> MAPKAKIVLVGSGMIGGVMATLIVQKNLGDVVLFDIVKNMPHGKALDTSHTNVMAYSNCKVSGSNTYDDLAGADVVIVTAGFTKAPGKSDKEWNRDDLLPLNNKIMIEIGGHIKKNCPNAFIIVVTNPVDVMVQLLHQHSGVPKNKIIGLGGVLDTSRLKYYISQKLNVCPRDVNAHIVGAHGNKMVLLKRYITVGG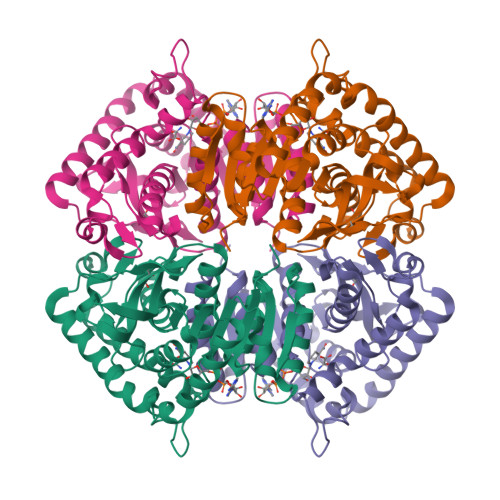IPLQEFINNKLISDAELEAIFDRTVNTALEIVNLHAAPYVAPAAAIIEMAESYLKDLKKVLICSTLLEGQYGHSDIFGGTPVVLGANGVEQVIELQLNSEEKAKFDEAIAETKRMKPLAHHHHHH> SGEQKMAEAHELLKKFYHHLLINTKEGQEALDYLLSRGFTKELINEFQIGYALDSWDFITKFLVKRGFSEAQMEKAGLLIRREDGSGYFDRFRNRVMFPIHDHHGAVVAFSGRALGSQQPKYMNSPETPLFHKSKLLYNFYKARLHIRKQERAVLFEGFADVISAVSSDVKESIATMGTSLTDDHVKILRRNVEEIILCYDSDKAGYEATLKASELLQKKGCKVRVAMI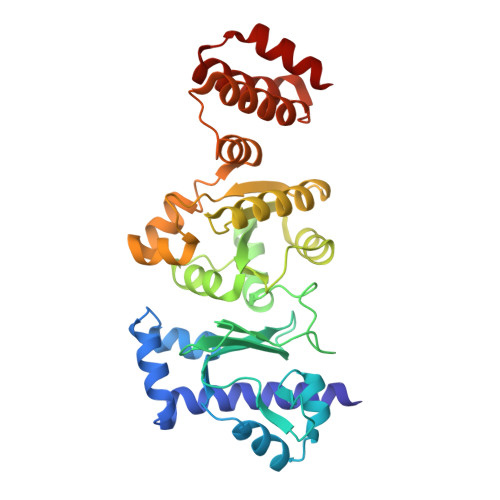PDGLDPDDYIKKFGGEKFKNDIIDASVTVMAFKMQYFRKGKNLSDEGDRLAYIKDVLKEISTLSGSLEQEVYVKQLASEFSLSQESLTEQLSVFS> GSMEGAGAGSGFRKELVSRLLHLHFKDDKTKVSGDALQLMVELLKVFVVEAAVRGVRQAQAEDALRVDVDQ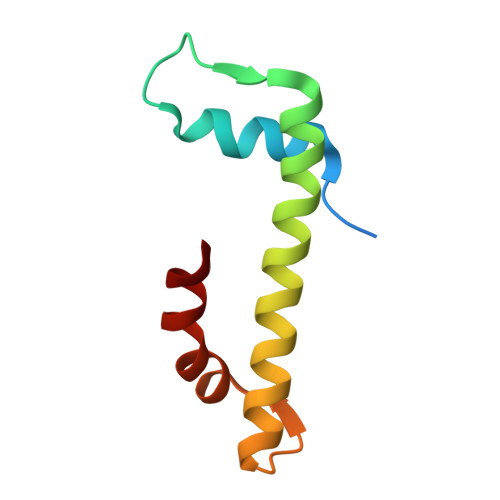LEKVLPQLLLDF>MDTILLTGLFAAFFTTFAFAPQSIKTIRTRNTEGISVVMYIMFLTGVISWIAYGIMRSDFAVLIANIVTLFLAAPVLVITLINRRKKHVLESSGENLYFQ[4x]

The SWEETs mediate the facilitative diffusion of sugars, by allowing solute permeation across biological membranes down a concentration gradient. SWEETs possess seven transmembrane (TM) helices, consisting of a pair of 3TM repeats and an additional helix that spans the membrane to connect these two repeats, resulting in the ‘3+1+3’ arrangement of TM helices. Their bacterial homologues, the SemiSWEETs, have only three TM helices. Previous studies have shown that the SemiSWEETs assemble into dimers to function as sugar transporters, and thus they are considered to be an ancestral form of the SWEETs.

We also obtained a crystal belonging to the different space group C2 (Crystal-II), and the structure was determined at 3.0 Å resolution by molecular replacement, using a protomer in Crystal-I as the search model. The asymmetric unit contains four EcSemiSWEET molecules organized into two separate dimers. Whereas the conformation of one dimer is almost identical to that of the inward-open state in Crystal-I, the other dimer adopts a markedly different conformation. In this alternative conformation, the extracellular halves of the protomers are separated from each other, while the intracellular halves approach the central axis. Consequently, the central cavity formed by the dimer is open towards the extracellular side. Hence, we designated this structure as the outward-open state. In the outward-open conformation, Phe19, Met39, Tyr40 and Phe43 of the two protomers form a cluster of aromatic and hydrophobic residues through van der Waals interactions. These interactions seal off the substrate-binding pocket from the intracellular environment. The temperature factors for the two conformations in Crystal-II implied that the outward-open conformation is inherently less stable than the inward-open conformation, suggesting that EcSemiSWEET probably prefers the inward-open conformation in the lipid environment. As the inward-open and outward-open conformations were simultaneously captured in Crystal-II in the absence of any sugars, the transition between these two conformations could spontaneously occur even without any substrates.4-[3-amino-6-(3,4,5-trimethoxyphenyl)pyrazin-2-yl]-2-methylbenzoic 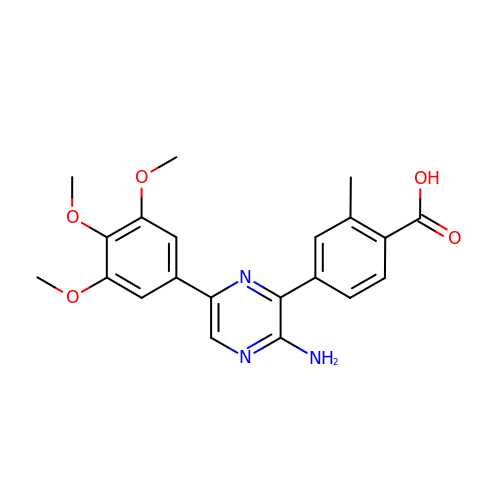acid | C21 H21 N3 O5 | AOAAZBKGFGSOFM-UHFFFAOYSA-N>MLFGRLTERAQRVLAHAQEEAIRLNHSNIGTEHLLLGLMKEPEGIAAKVLESFNITEDKVIEEVEKLIGHGQDHVGTLHYTPRAKKVIELSMDEARKLHHNFVGTEHILLGLIRENEGVAARVFANLDLNITKARAQVVKALGNPEMSNKNAQASKSNNTPTLDSLARDLTVIAKDGTLDPVIGRDKEITRVIEVLSRRTKNNPVLIGEPGVGKTAIAEGLAQAIVNNEVPETLKDKRVMSLDMGTVVAGTKYRGEFEERLKKVMEEIQQAGNVILFIDELHTLVGAGGAEGAIDASNILKPALARGELQCIGATTLDEYRKNIEKDAALERRFQPVQVDEPSVVDTVAILKGLRDRYEAHHRINISDEAIEAAVKLSNRYVSDRFLPDKAIDLIDEASSKVRLKSHTTPNNLKEIEQEIEKVKNEKDAAVHAQEFENAANLRDKQTKLEKQYEEAKNEWKNAQNGMSTSLSEEDIAEVIAGWTGIPLTKINETESEKLLSLEDTLHERVIGQKDAVNSISKAVRRARAGLKDPKRPIGSFIFLGPTGVGKTELARALAESMFGDDDAMIRVDMSEFMEKHAVSRLVGAPPGYVGHDDGGQLTEKVRRKPYSVILFDEIEKAHPDVFNILLQVLDDGHLTDTKGRTVDFRNTIIIMTSNVGAQELQDQRFAGFGGSSDGQDYETIRKTMLKELKNSFRPEFLNRVDDIIVFHKLTKEELKEIVTMMVNKLTNRLSEQNINIIVTDKAKDKIAEEGYDPEYGARPLIRA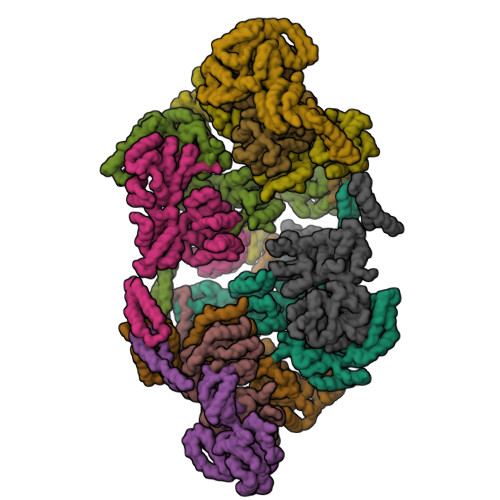IQKTIEDNLSELILDGNQIEGKKVTVDHDGKEFKYDIAEQTSETKTPSQA[10x]>[2x]MQEAARRASLRKEHTPTNEKFGDLSKQDSLGERASSKLTLDDELYDILYAFGETDAFINKGDKQRETDEDGNPLTRQALLERIRQKKEVIGKLRCQAWSMTRKRRTLKLAQKYLEQHESKVSRSHLYMEEMRKRARLMKRSFSNFKTYLIPWESKIKRIESHFGSVVSSYFTFLRWIVFVNIMITLIALVFVVLPETLADSVANEGRFNRTKTRKQIPANERVHADELAVVWHYDGYLRYSPLFYGYYSDDPFLGNKIKYALPLAYFMVTLTIFAYSFFAILRKMAANARMSKLSGSKAEQYIFNWKLFTGWDYTIGNSETASNTVMAVVIKLRESIADIKKDAHGKFRLLQFSLRVFANIIICAMLGFSIYCIIFAVQKSQVQDDGNLFTKNQVPSVVSTITHVFPMIFDLIGKMENYHPRTALRAHLGRVLILYTVNYITLIFALFEKMTALRDRVNSTSTSSSHRTKRQQGGWNPNMQRPPPYASRAEVRQMSDFLAANTRRFQTVSQRTTRSVTTPFTVAPQFGPFNVNNPNAVFHNGTHSTSFESQILGPKALPIFTPPPRKYPGFTPGNVGQQFGGPDFPRNQVYTKSTPLPRVRTKPPWVYTTTHPPLVQNRAMTTTMSKSAKKGNSKNLDDDILLSNETIQMSEAALRRNHDGHNNDICWETIIGQEIVKLVTMDLIFTILSILVIDLFRGLWIKYCSSWWCWDIETTFPEYGEFKVAENVLHIINNQGMIWLGLFFAPLLPAINNIKLIILMYIRGWAVMTCNVPAREIFRASRSSNFYLGILLIWLLLCTLPVGFVIASMSPSRSCGPFARYQHFYTVVTREIEKRVDQTVLSYIRHIASPGVVIPIILFLILIIYFLFSLVRGLREANTDLQAQLVHERTEEKKKIFELAGGKKNKFEKDRDKKRSNDYIPLIEQRRREPWRQYHEMEADHALASDSSEESDINEDEDDERQPLTAYPLRAIETPPETLQVTAFHPSLGSLIENREMEDEESASGDQLPMIHKSVSFQGPSHMQMRQSISTESCSQISRSAIQVATPEEIRALLRPYLEAKYGIPYQHGIKSFPIDVHTPPNNTPSRRSSKYNSFVSLYEHTRDDHKNFVASTIKETDEDPGKSDKKQTSSKDVAPDFMPWPSADEARALREKMKSKTPLMLTKTTVEEKPKGGKSSESEFRPPVPIHRKYNIQTTEEENEEEETDSAPESSKKRFRISVSPTKTIAPASASRAQHKIVSQASSSSSIPHGRQPDPNKKASLVLPPLRAPRVQFDEDDSPRQID;>MGNNASSLSELNLFSKGGVFTREQLDEYQDCTFFTRKDIIRLYKRFYALNPHKVPTNMQGNRPAITTLTFEEVEKMPELKENPFKRRICEVFSEDGRGNLSFDDFLDMFSVFSEMAPLQLKLKYAFRIYDYDGDELLGHDDLSKMIRSLTRDELSDVEVEFIIERIIEEADLDGDSSINFAEFEHVVSRSPDFIRTFHIRI[2x];>MPSGNEEINHLSALDQFVAPGLRLWMLIALVGGVLLIMIVIVCCFMRIRIPRTKRQIDLIAAKRKLRKSTKNSAEANAHNDERAQAIVMNSMPSGGGGGAPSTSSSRHTGSRIQSQV[2x]

Here we report the single-particle cryo-electron microscopy structure of the native transmembrane channel-like protein 1 (TMC-1) mechanosensory transduction complex isolated from Caenorhabditis elegans. The two-fold symmetric complex is composed of two copies each of the pore-forming TMC-1 subunit, the calcium-binding protein CALM-1 and the transmembrane inner ear protein TMIE. CALM-1 makes extensive contacts with the cytoplasmic face of the TMC-1 subunits, whereas the single-pass TMIE subunits reside on the periphery of the complex, poised like the handles of an accordion. Single-particle reconstructions and molecular dynamics simulations show how the mechanosensory transduction complex deforms the membrane bilayer and suggest crucial roles for lipid–protein interactions in the mechanism by which mechanical force is transduced to ion channel gating.

Two of these classes represent the TMC-1 complex in different conformational states, designated the ‘expanded’ (E) and ‘contracted’ (C) conformations, both of which exhibit an overall resolution of 3.1 Å. We observed a second conformation of the TMC-1 complex by 3D classification, designated as the C conformation. The TMC-1 subunits in the E and C conformations have a similar overall structure, both including closed ion channels. In the C conformation, however, the TM10 helix is bent approximately 9° compared with that in the E conformation, and there is one additional helical turn of TM10 in the E conformation. Upon successively superimposing the TMC-1 subunits from the C and E complexes, we observed that in the E state, each half of the TMC-1 complex, composed of TMC-1, CALM-1 and TMIE subunits, is rotated by around 8° compared with the C state, by way of an axis of rotation that is located near the TMC-1 H7 and H8 helices and oriented approximately parallel to the membrane. The movement of each half of the complex—when viewed parallel to the membrane plane—thus resembles the motion of an accordion, with the cytoplasmic regions of the complex undergoing relatively larger conformational displacements compared with those on the extracellular side of the membrane. Indeed, in comparing the C and E states, the amphipathic TMC-1 H3 helices move farther apart by approximately 11 Å, thus underscoring the magnitude of the conformational change. Nevertheless, these results illustrate the conformational plasticity of the TMC-1 complex and, reciprocally, the possibility that deformations of the membrane may induce conformational changes in the TMC-1 complex. Of note, the E and C conformations generate distinct membrane deformation patterns.> MQRSPLEKASVVSKLFFSWTRPILRKGYRQRLELSDIYQIPSVDSADNLSEKLEREWDRELASKKNPKLINALRRCFFWRFMFYGIFLYLGEVTKAVQPLLLGRIIASYDPDNKEERSIAIYLGIGLCLLFIVRTLLLHPAIFGLHHIGMQMRIAMFSLIYKKTLKLSSRVLDKISIGQLVSLLSNNLNKFDEGLALAHFVWIAPLQVALLMGLIWELLQASAFCGLGFLIVLALFQAGLGRMMMKYRDQRAGKISERLVITSEMIENIQSVKAYCWEEAMEKMIENLRQTELKLTRKAAYVRYFNSSAFFFSGFFVVFLSVLPYALIKGIILRKIFTTISFCIVLRMAVTRQFPWAVQTWYDSLGAINKIQDFLQKQEYKTLEYNLTTTEVVMENVTAFWEEGFGELFEKAKQNNNNRKTSNGDDSLFFSNFSLLGTPVLKDINFKIERGQLLAVAGSTGAGKTSLLMVIMGELEPSEGKIKHSGRISFCSQFSWIMPGTIKENIIFGVSYDEYRYRSVIKACQLEEDISKFAEKDNIVLGEGGITLSGGQRARISLARAVYKDADLYLLDSPFGYLDVLTEKEIFESCVCKLMANKTRILVTSKMEHLKKADKILILHEGSSYFYGTFSELQNLQPDFSSKLMGCDSFDQFSAERRNSILTETLHRFSLEGDAPVSWTETKKQSFKQTGEFGEKRKNSILNPINSIRKFSIVQKTPLQMNGIEEDSDEPLERRLSLVPDSEQGEAILPRISVISTGPTLQARRRQSVLNLMTHSVNQGQNIHRKTTASTRKVSLAPQANLTELDIYSRRLSQETGLEISEEINEEDLKECFFDDMESIPAVTTWNTYLRYITVHKSLIFVLIWCLVIFLAEVAASLVVLWLLGNTPLQDKGNSTHSRNNSYAVIITSTSSYYVFYIYVGVADTLLAMGFFRGLPLVHTLITVSKILHHKMLHSVLQAPMSTLNTLKAGGILNRFSKDIAILDDLLPLTIFDFIQLLLIVIGAIAVVAVLQPYIFVATVPVIVAFIMLRAYFLQTSQQLKQLESEGRSPIFTHLVTSLKGLWTLRAFGRQPYFETLFHKALNLHTANWFLYLSTLRWFQMRIEMIFVIFFIAVTFISILTTGEGEGRVGIILTLAMNIMSTLQWAVNSSIDVDSLMRSVSRVFKFIDMPTEGKPTKSTKPYKNGQLSKVMIIENSHVKKDDIWPSGGQMTVKDLTAKYTEGGNAILENISFSISPGQRVGLLGRTGSGKSTLLSAFLRLLNTEGEIQIDGVSWDSITLQQWRKAFGVIPQKVFIFSGTFRKNLDPYEQWSDQEIWKVADEVGLRSVIEQFPGKLDFVLVDGGCVLSHGHKQLMCLARSVLSKAKILLLDQPSAHLDPVTYQIIRRTLKQAFADCTVILCEHRIEAMLECQQFLVIEENKVRQYDSIQKLLNERSLFRQAISPSDRVKLFPHRNSSKCKSKPQIAALKEETEEEVQDTRL

pmcThe cystic fibrosis transmembrane conductance regulator (CFTR) is an anion channel expressed in the apical membrane of epithelial cells. Despite functioning as an ion channel, CFTR belongs to the superfamily of ATP-binding cassette (ABC) transporters. It is composed of two transmembrane domains (TMDs) and two nucleotide-binding domains (NBDs) that are common to all ABC transporters, along with a cytosolic regulatory (R) domain specific to CFTR. Once phosphorylated, adenosine triphosphate (ATP) binding promotes NBD dimerization and pore opening, whereas ATP hydrolysis leads to pore closure.

To identify the binding site of CFTRinh-172, we determined the cryo-EM structure of inhibitor-bound CFTR using phosphorylated CFTR (E1371Q). The structure was determined to an overall resolution of 2.7 Å. In the presence of CFTRinh-172 and ATP, CFTR (E1371Q) adopts an NBD-dimerized, pore-closed conformation distinct from any previously observed structures. The density for CFTRinh-172, as strong as the protein main chain atoms, was observed inside the pore, at a position corresponding to the membrane outer leaflet. CFTRinh-172 binds within the CFTR pore and interacts with both TMDs. The three rings of the compound form an elongated shape wedged between transmembrane helices (TMs) 1, 6, 8, 9, and 12. In the structure, the trifluoromethyl group fits snugly into a hydrophobic cavity, establishing van der Waals interactions with five hydrophobic residues on TMs 6, 8, 9, and 12. The carboxy group on CFTRinh-172 forms a salt bridge with K95. Furthermore, the anion selectivity filter (see accompanying paper) collapses, as TM1 undergoes a ~5° rotation that places the side chain of I106 at the position occupied by the chloride ion in the uninhibited structure. Our structural analysis clearly shows that binding of CFTRinh-172 leads to pore closure by trapping the TM helices in a non-conductive state.mithramycin | C52 H76 O24 | 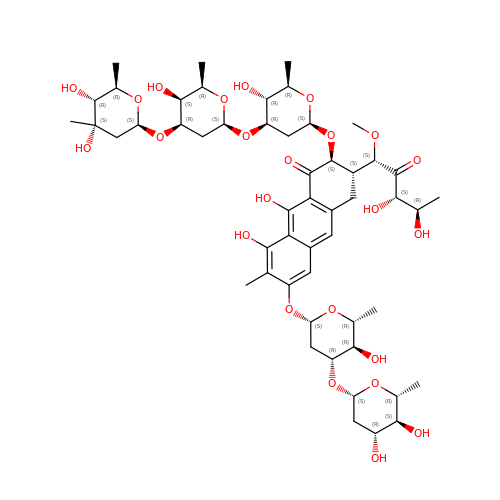CFCUWKMKBJTWLW-BKHRDMLASA-N> MSKESVRNDRNKKKKEPSKQECTESYEMTAELDDLTEKIRKAHQETFPSLCQLGKYTTNSSADHRVRLDLGLWDKFSELATKCIIKIVEFAKRLPGFTGLTIADQITLLKAACLDILILRICTRYTPEQDTMTFSDGLTLNRTQMHNAGFGPLTDLVFTFAN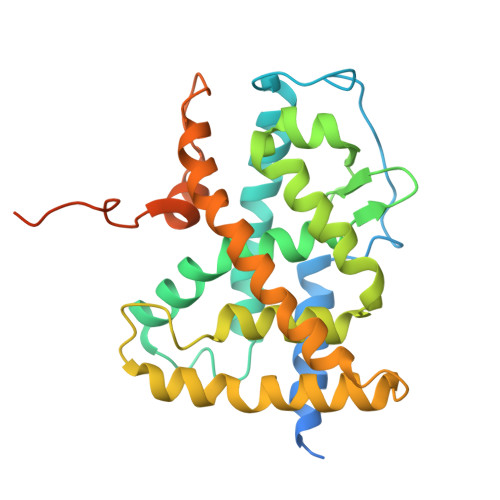QLLPLEMDDTETGLLSAICLICGDRQDLEEPTKVDKLQEPLLEALKIYIRKRRPSKPHMFPKILMKITDLRSISAKGAERVITLKMEIPGSMPPLIQEMLENSEGHEPLTPSSSGNIAEHSPSVSPSSVENSGVSQSPLLQ>MRGSHHHHHHGSMDKNIIIGAMTALITPFKNGKVDEQSYARLIKRQIENGIDAVVPVGTTGESATLTHEEHRTCIEIAVETCKGTKVKVLAGAGSNATHQAVGLAKFAKEHGADGILSVAPYYNKPTQQGLYEHYKAIAQSVDIPVLLYNVPGRTGCEISTDTIIKLFRDCENIYGVKEASGNIDKCVDLLAHEPRMMLISGEDAINYPILSNGGKGVISVTSNLLPDMISALTHFALDENYKEAKKINDELYNINKILFCESNPIPIKTAMYLAGLIESLEFRLPLCSPSKENFAKI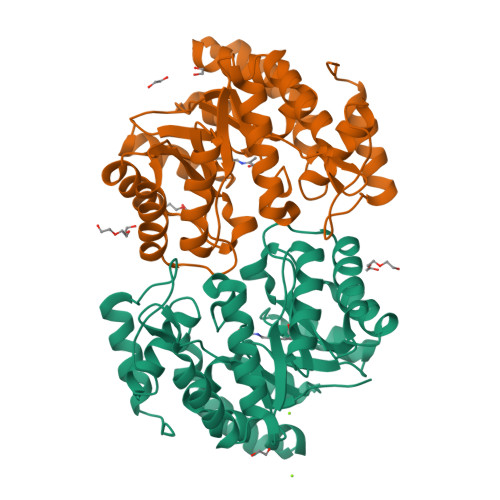EEVMKKYKIKGF[6x]> MTAINRRRFLQLFGAGAATAASSLAYGHAMHDSGNKAQRVVVIGGGFGGSTCARYLRHFDPDLEVTLINPSDTYTTCPFSNLVLGGERDLASITHDLSQLEHHHGVRLVQRWVESIDADGHRVVLDDGSAIGYDRLVVSPGIDLRWDAVEGYDQAAQEAMPHAWRPGEQTLLLRRQLEAMSDGGVVVIAPPANPFRCPPGPYERASLIAHYLKHHKPRSKILILDAKDAFAKQGL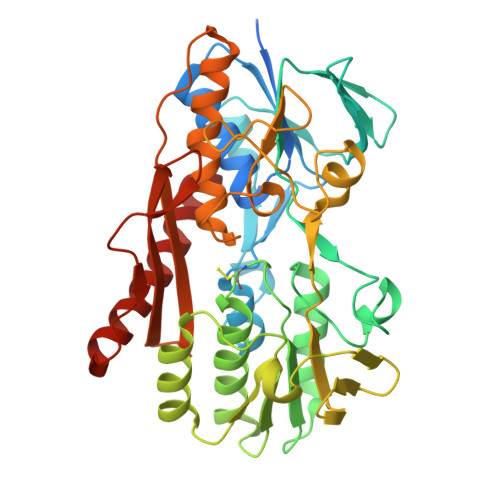FQTGWETLYPGMIEWVPGIEGGTVERVDAATGEVFTPSGRYRGDVVNLIPPQHAGAIARNTGLTDDSGWCPVNQQTFESLQIPHIHVIGDASIAGAMPKAGFAANSQAKVCAAAVVAALHGFDPTEPSWSSTCYSLVGPEYGISVSAVYRLDNGSIVASEGAGVSPGEADDHFRQLEAVYARGWYDNITAEMYG With regard to their common enzymatic activity, NDPKs are NTP/NDP transphosphorylases encoded by the nme genes. They catalyze the transfer of the γ-phosphate group from an NTP to an NDP via the formation of a high-energy intermediate on a catalytic histidine residue. We produced a truncated version of human NDPK isoform C (residues Thr18–Glu169, NDPK-C hereafter) and determined the 3D structure via X-ray crystallography in the absence and presence of various nucleotides. A data analysis revealed a hexameric arrangement, which is organized as three dimers, as previously reported for other functional eukaryotic NDPK variants.

Since this was not successful, we depleted the nucleotide from NDPK-C×UDP crystals by back soaking. The resolution of the corresponding structure was reduced to 2.64 Å, consistent with the idea that the nucleotide stabilizes the protein. Interestingly, we observed that the area where the phosphate groups in the nucleotide complex are located was occupied by a phosphate ion from the crystallization liquid and even formed a hydrogen bond to the imidazole ring of the catalytic histidine (His135). The residues involved in the interaction with phosphate are distinct for each subunit, but mostly Lys29 and Tyr69 play a role in stabilizing the phosphate. Moreover, the phosphate interacts via water molecules with Arg105 and Gly136 of all subunits inside the NDPK-C hexamer. In the absence of a nucleotide, the α2 helix and the Kpn-loop no longer tightly close off the active site of NDPK-C. The distance between Cα-Phe77 (one side of the gate) and Cα-Val129 (the opposite side of the gate) is changed from 10.2 Å in the complex with the nucleotide to 11.3 Å in the absence of UDP at the binding site. The removal of the UDP was accompanied by a small but detectable conformational change in the protein, particularly in the helices’ αA (from residue Ala60 to Arg73) and α2 (from residue Pro75 to Ser87) region. The B-factor values in this region are markedly higher upon nucleotide depletion, reflecting an increase in flexibility. Taken together, these data suggest that free phosphate in the active site of human NDPK-C likely mimics the phosphate in the transition state between the catalytic histidine and the γ-phosphate in the nucleoside triphosphate. Nevertheless, the electron densities of the residues that form a linker between the αA and α2 helices have disappeared in one trimer of apo NDPK-C. These data indicate that conformational changes in NDPK-C upon NDP removal can occur, with the helix α2 displaying the highest considerable shift in comparison with the nucleotide complexed protein.

>[6x]GHMTGAHERTFLAVKPDGVQRRLVGEIVRRFERKGFKLVALKLVQASEELLREHYAELRERPFYGRLVKYMASGPVVAMVWQGLDVVRTSRALIGATNPADAPPGTIRGDFCIEVGKNLIHGSDSVESARREIALWFRADELLCWEDSAGHWLYE>[2x]GSKKKIDILLKAVGDTPIMKTKKWAVERTRTIQGLIDFIKKFLKLV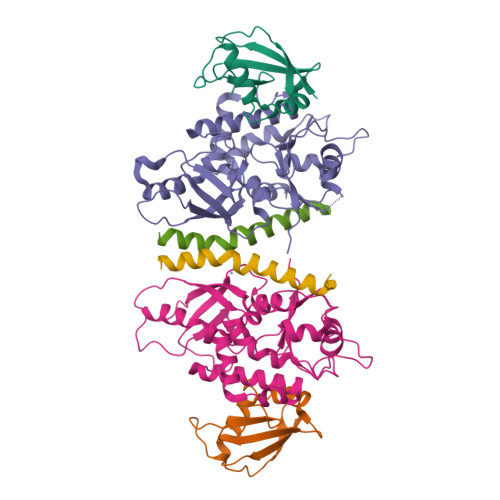ASEQLFIYVNQSFAPSPDQEVGTLYECFGSDGKLVLHYCKSQAWG;>MTDDKDVLRDVWFGRIPTCFTLYQDEITEREAEPYYLLLPRVSYLTLVTDKVKKHFQKVMRQEDISEIWFEYEGTPLKWHYPIGLLFDLLASSSALPWNITVHFKSFPEKDLLHCPSKDAIEAHFMSCMKEADALKHKSQVINEMQKKDHKQLWMGLQNDRFDQFWAINRKLMEYPAEENGFRYIPFRIYQTTTERPFIQKLFRPVAADGQLHTLGDLLKEVCPSAIDPEDGEKKNQVMIHGIEPMLETPLQWLSEHLSYPDNFLHISIIPQPTD[2x];>SHMPRWKRHISEQLRRRDRLQRQAFEEIILQYNKLL[2x]>SNAMNDIVASTQLPNTIKTITNDLRKLGLKKGMTVIVHSSLSSIGWISGGAVAVVEALMEVITEEGTIIMPTQSSDLSDPKHWSRPPVP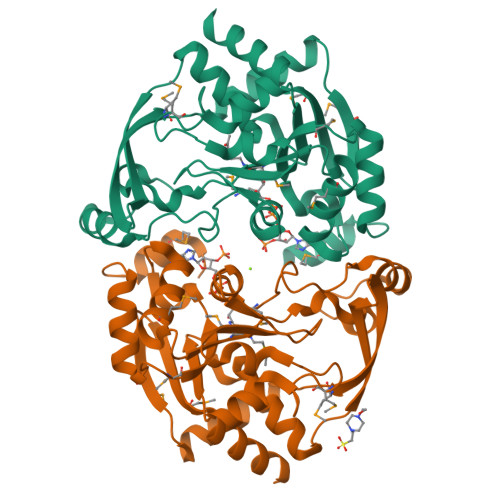EEWWQIIRDNVPAFEPHITPTRAMGKVVECFRTYPNVVRSNHPLGSFAAWGRHAEEITVNQSLSMSLGEESPLRKIYDLDGYILLIGVGYDSNTSVALSEVRSGACELIKVGAPIIENGERVWKEFVDMDYDSDKFVEIGVEFEQKGTVTMGKIGNAKCRLMKQRDIVDFGTEWFRKKN[4x]>[4x]MAHHHHHHSGTVTDDYLANNVDYASGFKGPLPMPPSKHIAIVACMDARLDVYRMLGIKEG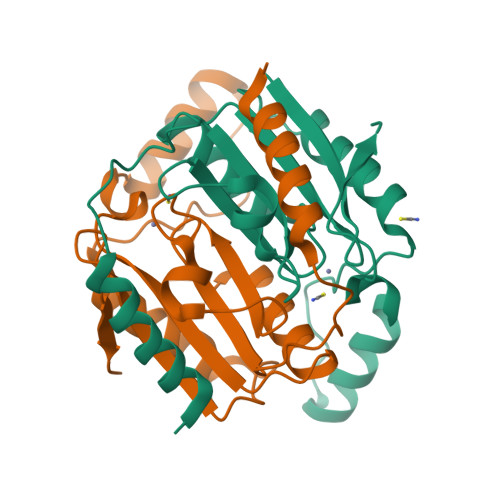EAHVIRNAGCVVTDDVIRSLAISQRLLGTREIILLHHTDCGMLTFTDDDFKRAIQDETGIRPTWSPESYPDAVEDVRQSLRRIEVNPFVTKHTSLRGFVFDVATGKLNEVTP> MAHHHHHHSAALEVLFQGPGPSPDELKPFPTVQQTIFRGHEGRVRSVAIDPTGVALATGGDDGTVRVWELLTGEQVWSVKLNGDEAVNTVRWRPTKDTFILAAAAGEDIFLMIPTHPSVTPALDQASRDILNAGFGHATNGKQQANLPPGKEPPGKWARPGTRLEDEGVLLRITVRSTIKAISWHRRGDHFATVSPSGQRSSVAIHTLSKHLTQIPFRKLNGLAQTASFHPLRPLFFVATQRSIRCYDLQKLELVKIVQPGAKWISSFD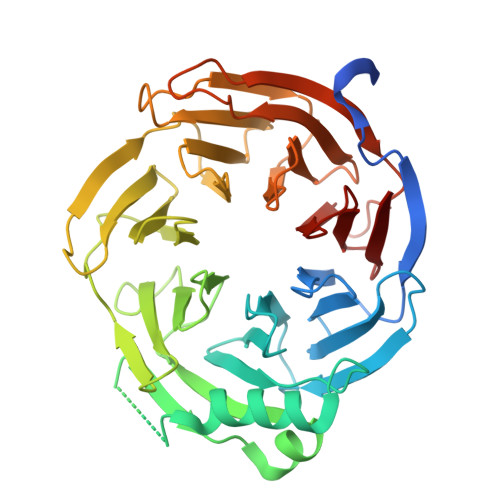VHPGGDNLVVGSYDKRLLWHDLDLSNRPYKTMRFHTEAIRAVRFHKGGLPLFADASDDGSLQIFHGKVPNDQLENPTIVPVKMLKGHKVVNKLGVLDIDWHPREPWCVSAGADGTARLWM>SMSWPSTVWHCFLKGTRLCFHKGSNKEWQDVEDFARAEGCDNEEDLQMGIHKGYGSDGLKLLSHEESVSFGESVLKLTFDPGTVEDGLLTVECKLDHPFYVKNKGWSSFYPSLTVVQHGIPCCEVHIGDVCLPPGHPDA[3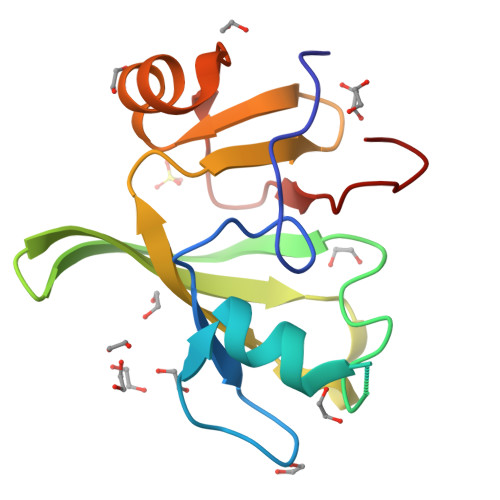x]> MKTKPLPTAPMAWAESAVETTTSPRELAGHAPLRRVLRPPIARRDGPVLLGDRAPRRTASTMWLLGIDPAESSPGTRATRDDTEQAVDKILRGARRAGGLTVPGAPRYHLTRQVTLTDLCQPNAERAGALLLALRHPTDLPHLARHRAPPGRQTERLAEAWGQLLE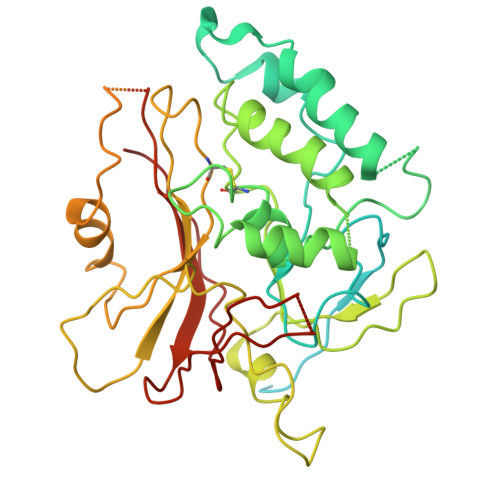ASALGSGRAESGCARAGLVSFNFLVAACAAAYDARDAAEAVRAHITTNYGGTRAGARLDRFSECLRAMVHTHVFPHEVMRFFGGLVSWVTQDELASVTAVCSGPQEATHTGHPGRPCSAVTIPACAFVDLDAELCLGGPGAAFLYLVFTYRQCRDQELCCVYVVKSQLPPRGLEAALERLFGRLRITNTIHGAEDMTPPPPNRNVDFPLAVLAASSQSPRCSASQVTNPQFVDRLYRWQPDLRGRPTARTCTYAAFAELGVMPDDSPRCLHRTERFGAVGVPVVILEGVVWRPGGWRACA>[3x]HGSP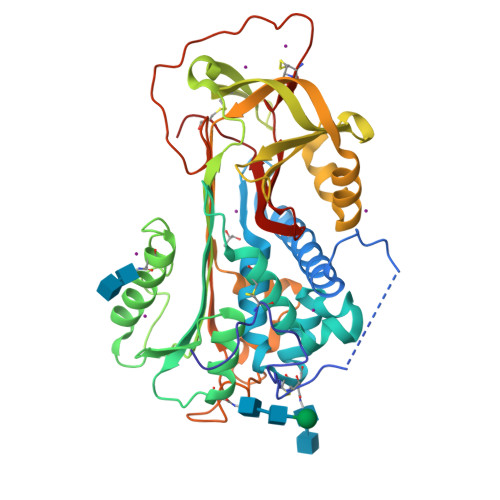VDICTAKPRDIPMNPMCIYRSPEKKATEDEGSEQKIPEATNRRVWELSKANSRFATTFYQHLADSKNDNDNIFLSPLSISTAFAMTKLGACNDTLQQLMEVFKFDTISEKTSDQIHFFFAKLNCRLYRKANKASKLVSANRLFGDKSLTFNETYQDISELVYGAKLQPLDFKENAEQSRAAINKWVSNKTEGRITDVIPSEAINELTVLVLVNTIYFKGLWKSKFSPENTRKELFYKADGESCSASMMYQEGKFRYRRVAEGTQVLELPFKGDDITMVLILPKPEKSLAKVEKELTPEVLQEWLDELEEMMLCVHMPRFRIEDGFSLKEQLQDMGLVDLFSPEKSKLPGIVAEGRDDLYVSDAFHKAFLEVNEEGSEAAASTAVVIAGRSLNPNRVCFKANRPFLVFIREVPLNTIIFMGRVANPCVK>MEKILIFGHQNPDTDTICSAIAYADLKNKLGFNAEPVRLGQVN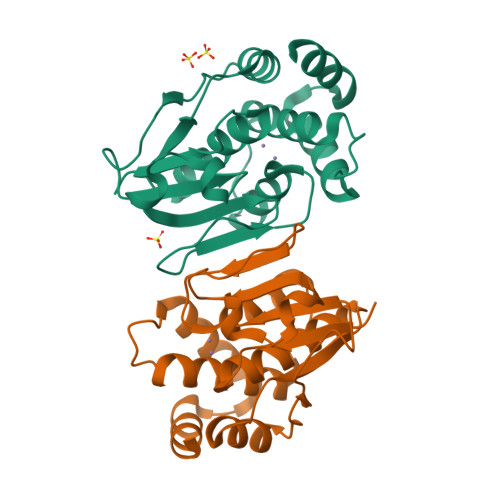GETQYALDYFKQESPRLVETAANEVNGVILVDHNERQQSIKDIEEVQVLEVIDHHRIANFETAEPLYYRAEPVGCTATILNKMYKENNVKIEKEIAGLMLSAIISDSLLFKSPTCTDQDVAAAKELAEIAGVDAEEYGLNMLKAG[2x]> MREYKLVVLGSGGVGKSALTVQFVQGIFVDEYDPTIEDSYRKQVEVDAQQCMLEILDTAGTEQFTAMRDLYMKNGQGFALVYSITAQSTFNDLQDLREQILRVKDTDDVPMILVGNKCDLEDERVVGKEQGQNLARQWNNCAFLESSAKSK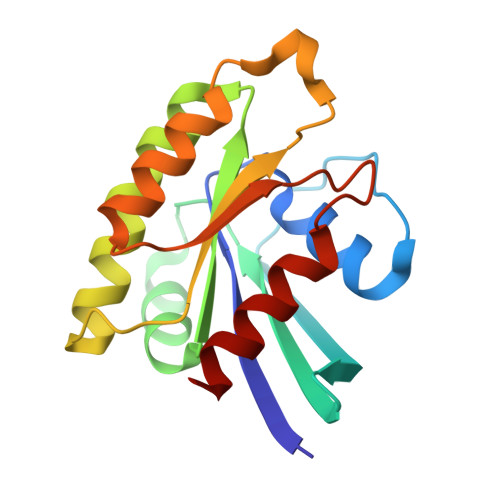INVNEIFYDLVRQINR> MSFESKKPMRTWSHLAEMRKKPSEYDIVSRKLHYSTNNPDSPWELSPDSPMNLWYKQYRNASPLKHDNWDAFTDPDQLVYRTYNLMQDGQESYVQSLFDQFNEREHDQMVREGWEHTMARCYSPLRYLFHCLQMSSAYVQQMAPASTISNCCILQTADSLRWLTHTAYRTHEL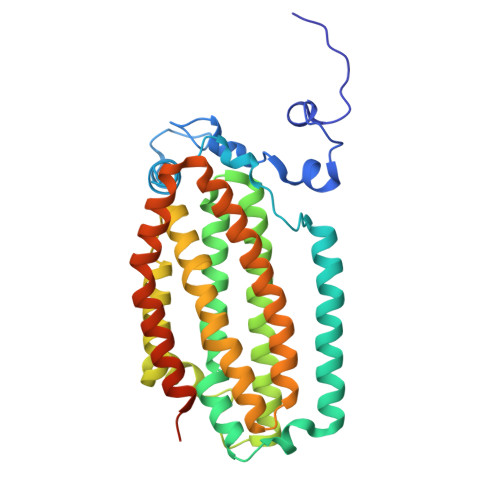SLTYPDAGLGEHERELWEKEPGWQGLRELMEKQLTAFDWGEAFVSLNLVVKPMIVESIFKPLQQQAYENNDTLLPLLIDSQLKDAERHSRWSKALVKHALENPDNHAVIEGWIEKWRPLADRAAEAYLSMLSSDILHAQYLERSTSLRASILTV> MGSSHHHHHHSSGLVPRGSMYLSKVIIARAWSRDLYQLHQGLWHLFPNR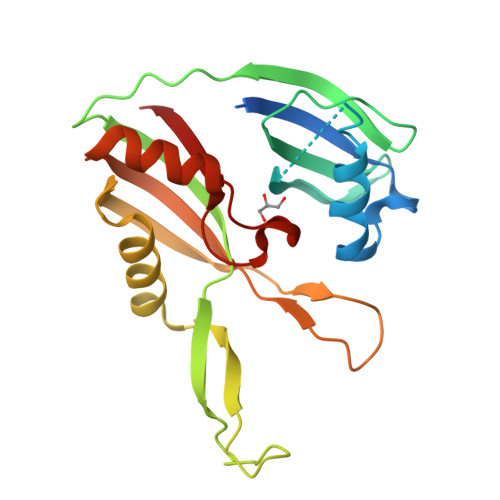PDAARDFLFHVEKRNTPEGCHVLLQSAQMPVSTAVATVIKTKQVEFQLQVGVPLYFRLRANPIKTILDNQKRLDSKGNIKRCRVPLIKEAEQIAWLQRKLGNAARVEDVHPISERPQYFSGDGKSGKIQTVCFEGVLTINDAPALIDLVQQGIGPAKSMGCGLLSLAPL>GHMHTPFIVALDFPSKQEVERFLRPFAGTPLFVKVGMELYYQEGPAIVAFLKEQGHAVFLDLKLHDIPNTVKQAMKGLARVGADLVNVHAAGGRRMMEAAIEGLDAGTPSGRMRPRCIAVTQLTSTDERMLHEELW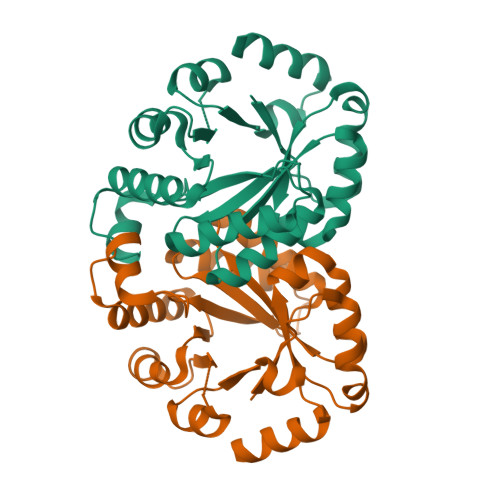ISRPLVETVAHYAALAKESGLDGVVCSANEAAFIKERCGASFLAVTPGIRFADDAAHDQVRVVTPRKARALGSDYIVIGRSLTRAADPLRTYARLQHEWNGGERESTTPT[4x]> CGUGGUUAGGGCCACGUUAAAUAGUUGCUUAAGCCCUAAGCGUUGAU;> AUCAGGUGC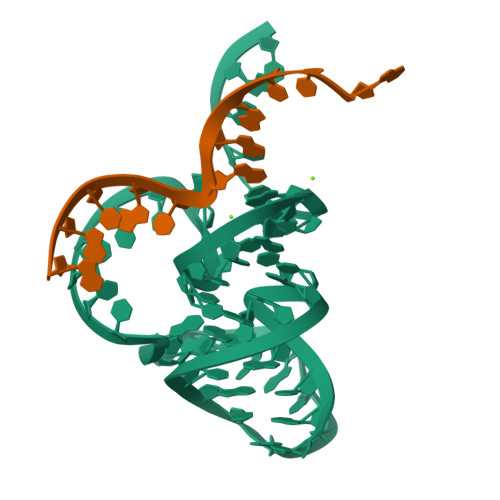AA>[4x]MSLNEKVALVTGASRGIGFEVAHALASKGATVVGTATSQASAEKFENSMKEKGFKARGLVLNISDIESIQNFFAEIKAENLAIDILVNNAGITRDNL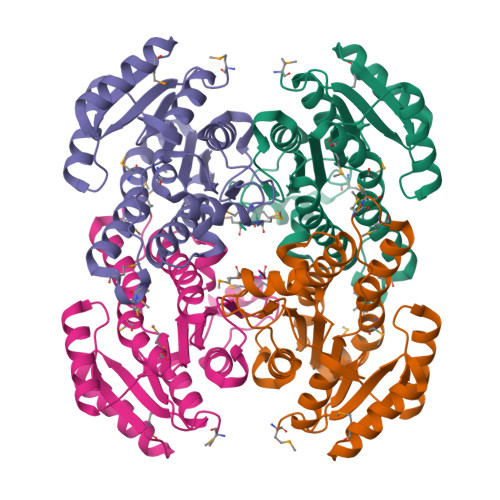MMRMSEDEWQSVINTNLSSIFRMSKECVRGMMKKRWGRIISIGSVVGSAGNPGQTNYCAAKAGVIGFSKSLAYEVASRNITVNVVAPGFIATDMTDKLTDEQKSFIATKIPSGQIGEPKDIAAAVAFLASEEAKYITGQTLHVNGGMYMA> MLYIDEFKEAIDKGYILGDTVAIVRKNGKIFDYVLPHEKVRDD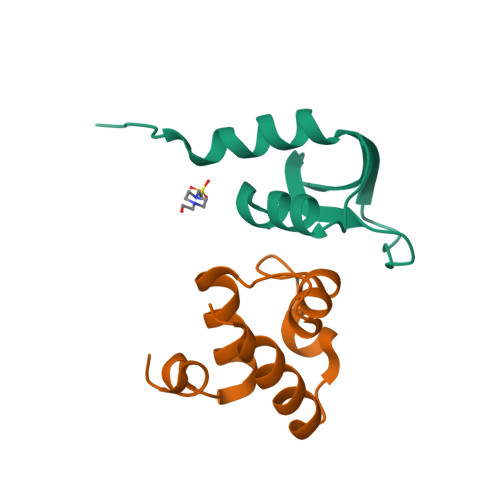EVVTVERVEEVMVELDKLEHHHHHH;> MLKDFGKKIKSLRLEKGLTKEAVCLDESQLSTRQLTRIESGQSTPTLNKAVYIAGRLGVTLGYLTDGE> NGDRLYRADSRPPDEIKRSGGLMPRGHNEYFDRGTQMNINLYDHARGTQTGFVRYDDGYVSTSLSLRSAHLAGQSILSGYSTYYIYVIATAPNMFNVNDVLGVYSPHPYEQEVSALGGIPYSQIYGWYRVNFGVIDERLHRNREYRDRYYRNLNIAPAEDGYRLAGFPPDHQAWREEPWIHHAP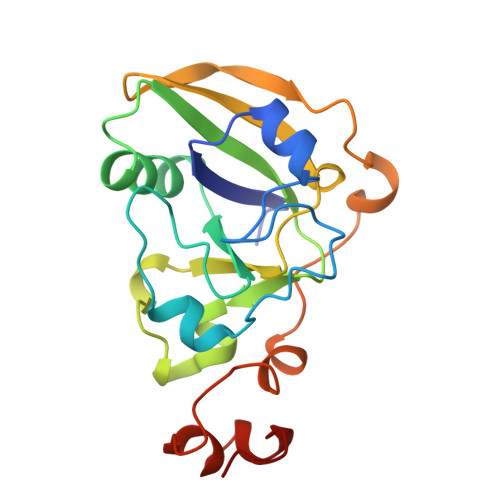QGCG>SQQQIAALSESLQATQQQLQALQQQCYELEKTNRL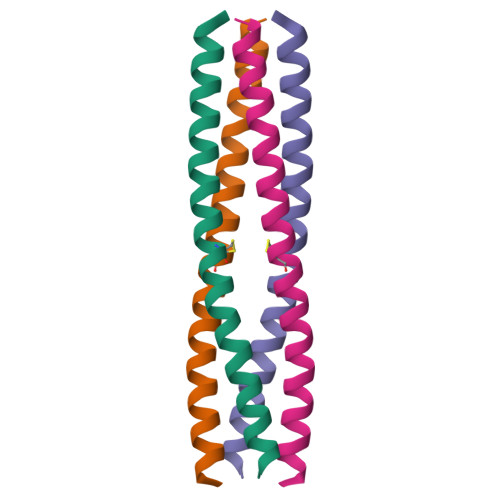LVSEVMTLQKMVKAQ[2x]> MATDGLHENETLASLKSEAESLKGKLEEERAKLHDV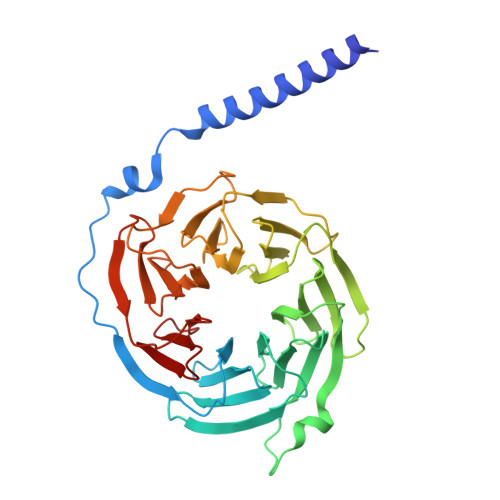ELHQVAERVEALGQFVMKTRRTLKGHGNKVLCMDWCKDKRRIVSSSQDGKVIVWDSFTTNKEHAVTMPCTWVMACAYAPSGCAIACGGLDNKCSVYPLTFDKNENMAAKKKSVAMHTNYLSACSFTNSDMQILTASGDGTCALWDVESGQLLQSFHGHGADVLCLDLAPSETGNTFVSGGCDKKAMVWDMRSGQCVQAFETHESDVNSVRYYPSGDAFASGSDDATCRLYDLRADREVAIYSKESIIFGASSVDFSLSGRLLFAGYNDYTINVWDVLKGSRVSILFGHENRVSTLRVSPDGTAFCSGSWDHTLRVWA>MAEKIPKPVSKRLVSYYMCLERLLDEGVEVVSSEELARRLDLKASQIRKDLSYFGEFGKRGVGYNVEHLYDAIGEILGVKKEWKLVVVGAGNIGRAVANYTVMKEKGFRIIGIFDSDPSKIGKEAAPGLTVSDVSEL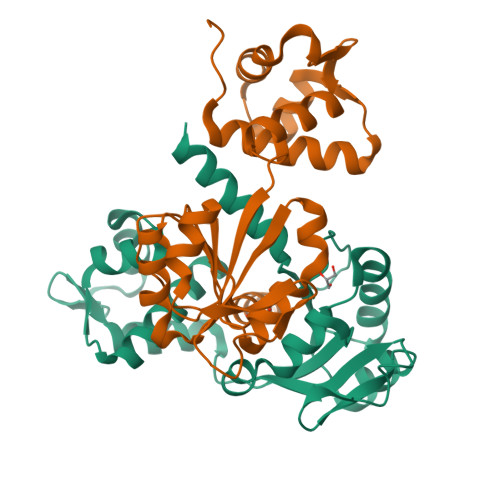EKFVEEHGVEIGVIAVPAEHAQEIAERLEKAGIKGILNFAPVKIKVSVPVENIDITASLRVLTFEIVRRNS[4x]(2S,3R,4R,5S,6R)-3-AMINO-4-({[(2S,3R,4R,5S,6R)-3-AMINO-2-{[(1R,2R,3S,4R,6S)-4,6-DIAMINO-2,3-DIHYDROXYCYCLOHEXYL]OXY}-5-HYDROXY-6-(HYDROXYMETHYL)TETRAHYDRO-2H-PYRAN-4-YL]OXY}METHOXY)-6-(HYDROXYMETHYL)TETRAHYDRO-2H-PYRAN-2,5-DIOL 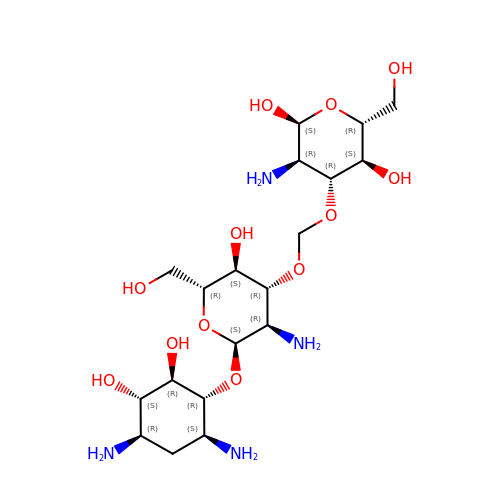| C19 H38 N4 O12 | BKAACSMFIQVWGC-LZHQQFSOSA-N>[2x]GSHMRFYVKDHRN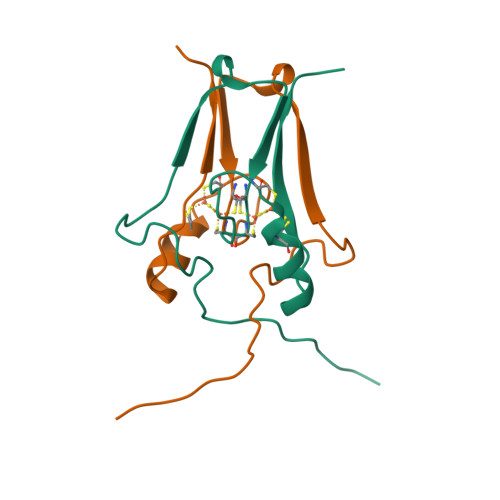KAMINLHIQKDNPKIVHAFDMEDLGDKAVYCRCWRSKKFPFCDGACTKHNEETGDNVGPLIIKKKE>MAKDPRYVGNLPKIGIRPTIDGRRKGVRESLEETTMNMAKAVAKLLEENVFYYNGQPVECVIADTCIGGVKEAAEAAEKFAREGVGVSITVTPCWCYGTETMDMDPHIPKAVWGFNGTERPGAVYLAAVLAGYNQKGLPAFGIYGKDVQDAGDTNIPEDVKEKL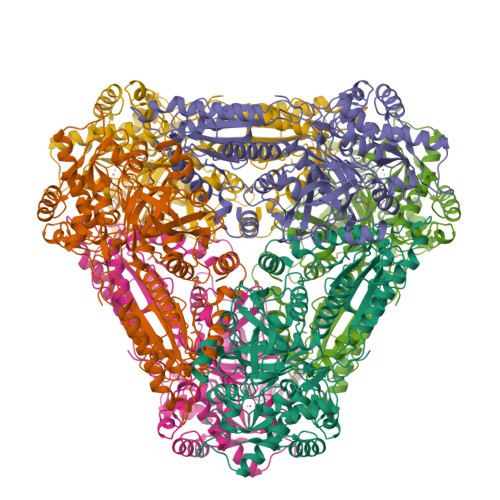IRFAKAGLAVAMMKGKSYLSIGSVSMGIAGSVVQEDFFQNYLGMRNEYVDMSEFVRRIELGIYDKEEYERALKWVKENCKVGPDNNRDGFKRTEEQKEKDWEISVKMALIARDLMVGNKKLEEMGYGEEALGRNAIVAGFQGQRQWTDYFPNGDFMETILNSSFDWNGKRAPYIFATENDNLNGISMLFGYLLTNTAQIFADVRTYWSPEAVKRVTGYTLEGRAANGIIHLINSGAAALDGTGEQTKDGKPVIKPYYELTDEDIKKCLEATQFRPASTEYFRGGGYSTDFLTKGGMPVTISRLNIVKGLGPVLQIAEGYTVDLPEEVHDVLDKRTDPTWPTTWFVPNLTGEGAFKDVYSVMNNWGANHCSISYGHIGADLITLASILRIPVNMHNVPEEKIFRPDAWSMFGTKDLEGADYRACKKLGPIYK[3x]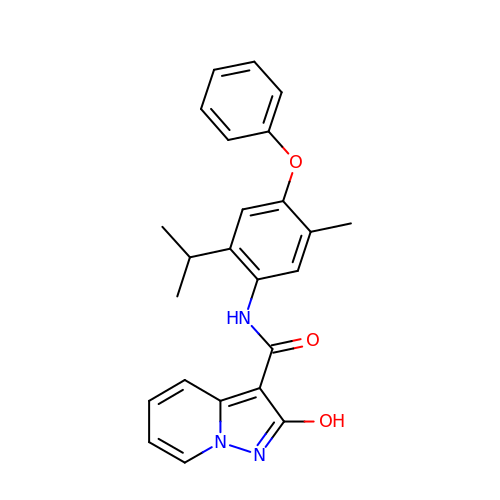~{N}-(5-methyl-4-phenoxy-2-propan-2-yl-phenyl)-2-oxidanyl-pyrazolo[1,5-a]pyridine-3-carboxamide | C24 H23 N3 O3 | JABKJLQKEVJGOT-UHFFFAOYSA-N>KHSLPDLPYDYGALEPHINAQIMQLHHSKHHAAYVNNLNVTEEKYQEALAKGDVTAQTALQPALKFNGGGHINHSIFWTNLSPNGGGEPKGELLEAIKRDFGSFDKFKEKLTAASVGVQGSGWGWLGFNKERGHLQIAACPNQDPLQGTTGLIPLLGIDVWEHAYYLQYKNVRPDYLKAIWNVINWENVTERYMACKK[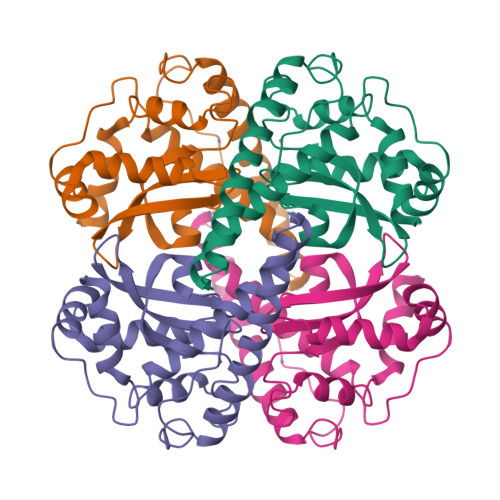2x]> MGHHHHHHGSVKIGHYILGDTLGVGTFGKVKVGKHELTGHKVAVKILNRQKIRSLDVVGKIRREIQNLKLFRHPHIIKLYQVISTPSDIFMVMEYVSGGELFDYICKNGRLDEKESRRLFQQILSGVDYCHRHMVVHRDLKPENVLLDAHMNAKIADFGLSNMMSDGEFLRTSCGSPNYAAPEVISGRLYAGPEVDIWSSGVILYALLCGTLPFDDDHVPTLFKKICDGIFYTPQYLNPSVISLLKHMLQVDPM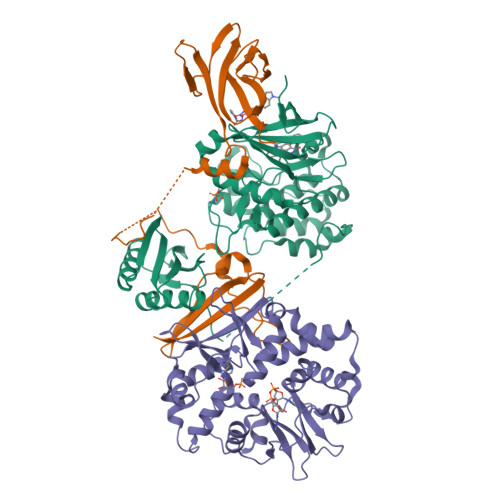KRATIKDIREHEWFKQDLPKYLFPEDPSYSSTMIDDEALKEVCEKFECSEEEVLSCLYNRNHQDPLAVAYHLIIDNRRIMNEAKDFYLATSPPDSFLDDHHLTRPHPERVPFLVAETPRARHTLDELNPQKSKHQGVRKAKWHLGIRSQSRPNDIMAEVCRAIKQLDYEWKVVNPYYLRVRRKNPVTSTYSKMSLQLYQVDSRTYLLDFRSIDDELTPRPGSHTIEFFEMCANLIKILAQ;> MEVNDKAPAQARPTVFRWTGGGKEVYLSGSFNNWSKLPLTRDHNNFVAILDLPEGEHQYKFFVDGQWTHDPSEPIVTSQLGTVNNIIQVKKTDFEVFDALMVDSQKCSDVSELSSSPPGPYHQEPYVCKPEERFRAPPILPPHLLQVILNKDTGISCDPALLPEPNHVMLNHLYALSIKDGVMVLSATHRYKKKYVTTLLYKPI;> METVISSDSSPAVENEHPQETPESNNSVYTSFMKSHRCYDLIPTSSKLVVFDTSLQVKKAFFALVTNGVRAAPLWDSKKQSFVGMLTITDFINILHRYYKSALVQIYELEEHKIETWREVYLQDSFKPLVCISPNASLFDAVSSLIRNKIHRLPVIDPESGNTLYILTHKRILKFLKLFITEFPKPEFMSKSLEELQIGTYANIAMVRTTTPVYVALGIFVQHRVSALPVVDEKGRVVDIYSKFDVINLAAEKTYNNLDVSVTKALQHRSHYFEGVLKCYLHETLETIINRLVEAEVHRLVVVDENDVVKGIVSLSDILQALVLTGGEKKP>MAASYNDHNHLASGESKSQIVVVMVPFPAQSHLNQLLHLSRLISPYNIPIHYVSTPSHVRQAKSRLQNWNINSATNFHIHEYPIPSFEALPPNPNDPTKFPTHLLPLFHASRHLCEPVTALLHSLAATAHRVVVIHDVLISSVVQEVKNIPNAEAYALQSVSVFNHFATIWEMMGKPSSVEDEALNHLPSQEGCVPMEFIEILMSQSHLANQFATGFIHNTSKAIEGKYVDFLDKEEFSGNIKQWALGPFNPVSVSNEEKIRHKCLNFLDKQSPRSVMYVSFGTTISFTDEQIHELALGLEKSEQHFIWVLREADRGDIYAGTERKTELPNGYEDRIKEKGMMVRDWVPQLEILAHPSTGGFMSHCGWNSCLDSLTMGVPVAAWPMHSDQP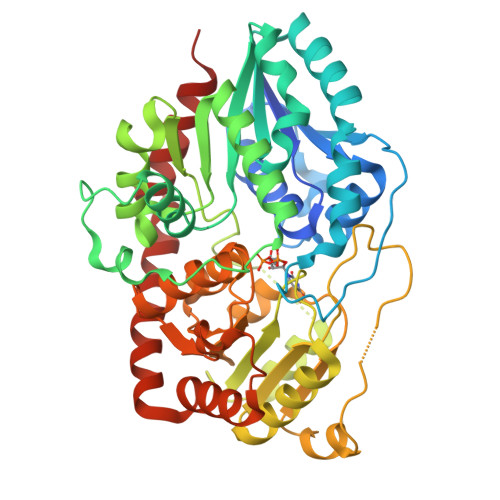RNAMLVVDVLKIGTFVNDWEKRSELVSSAMIAKAVKKLVASKEGAEIRKRAVEMGAAVRQSVADGGVTRMELDSFIAQISRI[2x]>[8x]MSQSVSERTRIKSDRYESGVIPYAKMGYWDAAYSVKDTDVLALFRITPQPGVDPVEAAAAVAGESSTATWTVVWTDLLTACERYRAKAYRVDPVPNSTDVYFAFIAYECDLFEEASLSNLTASIIGNVFGFKAISALRLEDMRIPHSYLKTFQGPATGIIVE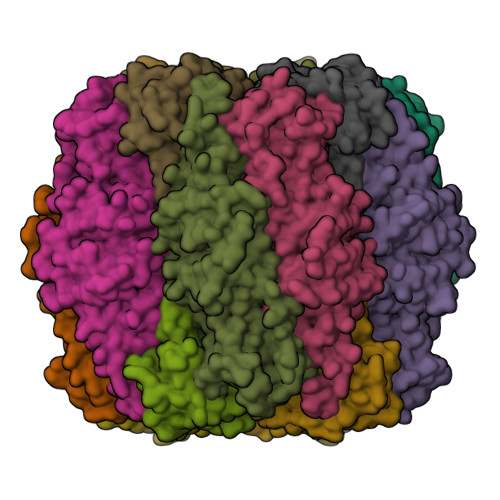RERLNKYGTPLLGATVKPKLGLSGKNYGRVVYEGLKGGLDFLKDDENINSQPFMRWRERFLNCLEGINRAAAATGEVKGSYLNITAATMEEVYKRAEYAKAIGSVVVMIDLVMGYTAIQSIAYWARENDMLLHLHRAGNSTYARQKNHGINFRVICKWMRMSGVDHIHAGTVVGKLEGDPLMIKGFYDVLRLTELEVNLPFGIFFEMDWASLRRCMPVASGGIHCGQMHQLIHYLGDDVVLQFGGGTIGHPDGIQAGATANRVALEAMVLARNEGADYFNNQVGPQILRDAAKTCGPLQTALDLWKDISFNYTSTDTADFAETATANR;>MRLTQGCFSFLPDLTDQQIEKQVTYAMNRGWAMNVEWTDDPHPRNNYWELWGLPLFDIKDPATVMFELNEARKSCAAGYIRVNAFDASYGTESCVMSFITNRPANEPGFYLDRTEGVGRQVIYSIKSYSVQANPEGSRY[8x]3 bromo 4 hydroxybenzoic acid | C7 H5 Br O3 | 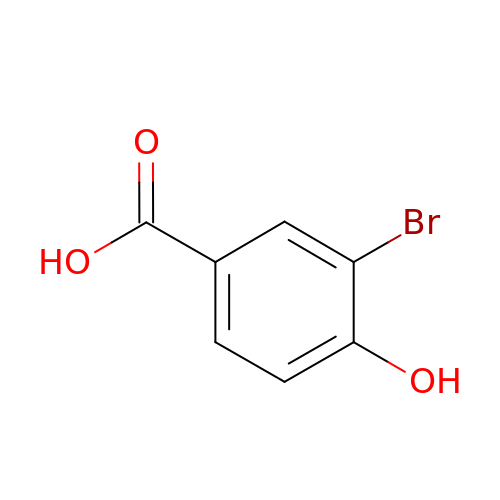XMEQDAIDOBVHEK-UHFFFAOYSA-N> MTMASVPASRYLTDMTLEEMSRDWSMLIPKQKVAGPLCIRMDQAIMDKNIILKANFSVIFDRLETLILLRAF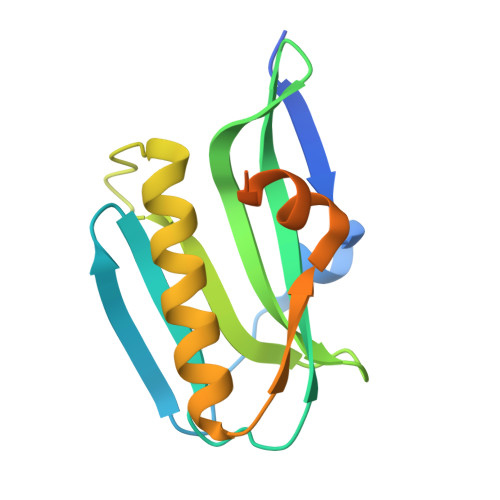TEEGAIVGEISPLPSLPGHTAEDVKNAVGVLIGGLEANDNTVRVSETLQRFAWRSSNENGRPPLTPKQKREMAGTIRSEV> MNPFHELEPGPEVPEVVYALIEIPKGSRNKYELDKATGLLKLDRVLYSPFFYPVDYGIIPQTWYDDGDPFDIMVIMREPVYPLTIIEARPIGIMKMED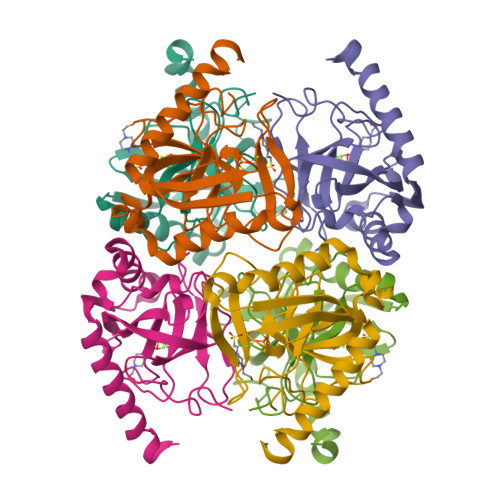SGDKDWKVLAVPVEDPYFNDWKDISDVPKAFLDEIAHFFQRYKELQGKTTKIEGWGNAEEAKREILRAIEMYKEKFGKEE The traditional immunomodulatory drugs (IMiDs) such as thalidomide and its analogues (all based on the phthalimide glutarimide core) bind to Cereblon, the substrate receptor of the CRL4ACRBN E3 ligase. The binding mode of thalidomide includes a hydrogen bond between one of the phthalimide carbonyl groups and a conserved asparagine residue of the protein, which contributes to the affinity between the two molecules. However, the other phthalimide carbonyl is not involved in any specific interactions, not even with water molecules, and thus represents an unsatisfied polar group that potentially lowers the binding energy.

We hypothesised that replacing the phthalimide core with benzotriazole, thereby removing both carbonyl groups, would possibly eliminate the possibility of hydrogen bonding with the conserved asparagine, but also rid the molecule of the “dissatisfied” carbonyl group. As the net result, the affinity to CRBN may be retained, assuming that the introduced triazole nitrogen is less unfavoured than the carbonyl group due to its decreased polarity with only a single free electron pair. We designed a thalidomide analogue in which the phthalimide moiety was replaced with benzotriazole, using an innovative synthesis strategy. To our delight, when evaluated for affinity to the thalidomide-binding domain of human CRBN in comparison to thalidomide (1, Ki 8.5 ± 0.8 µM), using the recently reported thermophoresis-based assay, the benzotriazolo analogue 2 displayed an improvement in affinity with a Ki value of 6.8 ± 1.6 µM. To gain insight into the binding mode of 2, we employed our previously established crystal soaking system based on the bacterial CRBN homologue Magnetospirillum gryphiswaldense Cereblon Isoform 4 (MsCI4). The obtained crystal structure revealed that 2 binds in the same overall orientation as thalidomide, but lacks any specific hydrogen-bonding interactions with the target other than those mediated by the glutarimide moiety. None of the benzotriazole nitrogen is involved in hydrogen bonds, not even to water, suggesting that the retained affinity could indeed be due to their lower polarity as compared to the ‘unsatisfied’ carbonyl groups in thalidomide. Despite the absence of the carbonyl group involved in hydrogen bonding with CRBN, it retained affinity, likely due to the relief from the other, ‘dissatisfied’ carbonyl group. These assumptions are corroborated by the crystal structure of the complex between 2 and CRBN.

>AMPLDAGGQNSTQMVLAPGASIFRCRQCGQTISRRDWLLPMGGDHEHVVFNPAGMIFRVWCFSLAQGLRLIGAPSGEFSWFKGYDWTIALCGQCGSHLGWHYEGGSQPQTFFGLIKDRLAEGPAD[3x]>MDKKGSDSGKASGEQVLNLTESALIPSADSTKADDQVGLNVVNQTNEGLYALDKDGIPAIAGAAEEPKISDDKTVYTIKLREDAKWSNGDPVTANDYVYSWRRAVDPNTAATYSYLFDAIKNGGDIVAGKKKPEELGIKAVDDYTLEVTLSKPTAYINSLFAFPTFFPLNEKFVTEKGEKYAQNSDNMLFNGPFELKDWTGTNKKWTYVKNDKYWDKDKVKLKQINVQVVQDSGTGLNLYNTDKVDRTVLSADYAAQNKNNKDYVTVNNSSTFYIKFNQKRAGKDTVFANKNIRKAIALAIDKQSYTDTVLKNGSKPANNLVPEGFTFD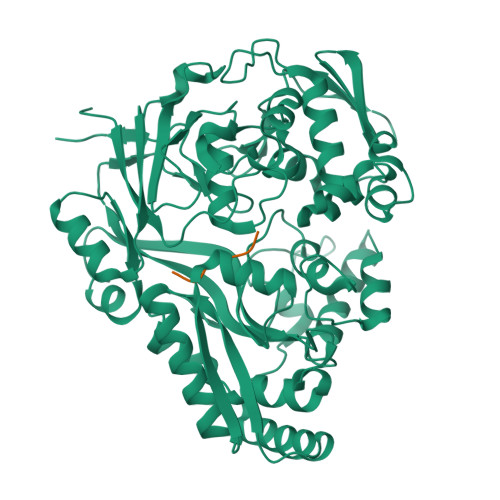PGNKEDYTKESGKHLEYDVKEAQKAWKAGLKELGVNEITVEFTSDDTENARKSSEFIQDQLQKNLDGLTVKLKNVPFKVRLQNDQNQDYDFSMSGWGPDYQDPSTFLDLFVTDGAQNRMSYSNKDYDKILNDASVTYAADDQKRWDEMVKAEKILLTDDVAIQPLYQRSTAYLQKDYIKNLQKNPFGPDYTYKETYLTKLEHHHHHH[2x];> SDESKG;> SDESSG>[5x]MTDMNILDLFLKASLLVKLIMLILIGFSIASWAIIIQRTRILNAAAREAEAFEDKFWSGIELSRLYQESQGKRDNLTGSEQIFYSGFKEFVRLHRANSHAPEAVVEGASRAMRISMNRELENLETHIPFLGTVGSISPYIGLFGTVWGIMHAFIALGAVKQATLQMVAPGIAEALIATAIGLFAAIPAVMAYNRLNQRVNKLELNYDNFMEEFTAILHRQAFTVSESNKG;>[2x]MARARGRGRRDLKSEINIVPLLDVLLVLLLIFMATAPIITQSVEVDLPDATESQAVSSNDNPPVIVEVSGIGQYTVV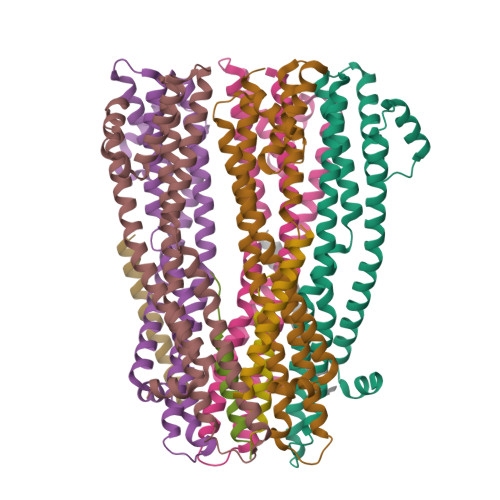VEKDRLERLPPEQVVAEVSSRFKANPKTVFLIGGAKDVPYDEIIKALNLLHSAGVKSVGLMTQPI;>[3x]MSKATEQNDKLKRAIIISAVLHVILFAALIWSSFDENIEASAGGGGGSSIDAVMVDSGAVVEQYKRMQSQESSAKRSDEQRKMKEQQAAEELREKQAAEQERLKQLEKERLAAQEQKKQAEEAAKQAELKQKQAEEAAAKAAADAKAKAEADAKAAEEAAKKAAADAKKKAEAEAAKAAAEAQKKAEAAAAALKKKAEAAEAAAAEARKKAATEAAEKAKAEAEKKAAAEKAAADKKAAAEKAAADKKAAEKAAAEKAAADKKAAAEKAAADKKAAAAKAAAEKAAAAKAAAEADDIFGELSSGKNAPKTGGGAKGNNASPAGSGNTKNNGASGADINNYAGQIKSAIESKFYDASSYAGKTCTLRIKLAPDGMLLDIKPEGGDPALCQAALAAAKLAKIPKPPSQAVYEVFKNAPLDFKP>MMVWKVLIADDEAIIREGIRESIDWNEFNMEVVAEAEDGEEALELALRHRVDVLFVDLSMPIMDGLTLMKYAREKLPNCHMIVITGYDEFSYAQ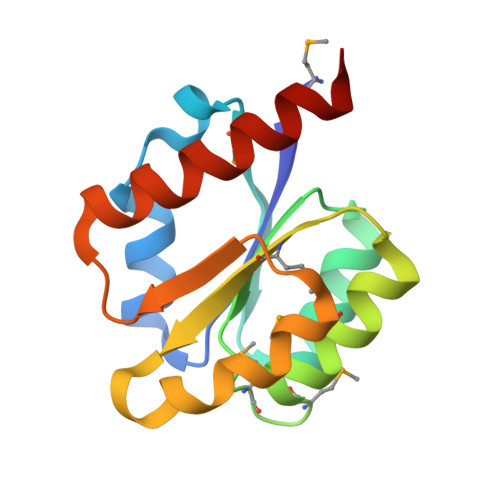EAIRLQVDDYLLKPTDPQRLREVVAKVKEKLEQEQKEK[2x]Replication Protein A (RPA) is a heterotrimeric single stranded DNA-binding protein with essential roles in DNA replication, recombination and repair. In Archaea, the same function is also fulfilled by a heterotrimeric RPA. We report three crystal structures and five cryo-EM structures of Pyrococcus abyssi RPA (hereafter referred to PabRPA), in its apo form as well as bound to ssDNA. We find that archaeal and eukaryotic RPAs share a conserved heterotrimerization core, which is composed of three OB domains connected through a three-helix bundle formed by a C-terminal α-helix from each subunit.

We also collected two independent cryo-EM SPA (single-particle analysis) datasets showing multiple PabRPAs coating the ssDNA by using a poly-dT100 oligonucleotide. Interestingly, 2D class averages reveal that PabRPA dimers adopt two different conformations in the two datasets. In the second dataset, PabRPA-ssDNA complexes are more condensed, adopting a pseudo-helicoidal configuration. 2D class averages show additional density for OB-1 that connects two Tri-Cs from adjacent RPAs. Both 3D reconstructions show that two PabRPA molecules interact with each other on ssDNA through the OB-1 domain of one PabRPA that packs against the Tri-C of an adjacent PabRPA protomer particularly with its OB-4 domain. While their OB-1 domains are similarly oriented in both types of oligomeric forms, the OB-1 domain is more loosely packed to the adjacent Tri-C in the relaxed form than in the condensed one. Differences between the two DNA-bound PabRPA oligomeric forms are due to a rotation around the OB-1/OB-2 domains of the Rpa1 subunit. In the condensed PabRPA filament, this rotation brings RPA protomers closer together, compared to their position in the relaxed linear filaments observed in PabRPA and SceRPA17. Importantly, in both types of filaments, the DNA-binding groove of OB-1 is ideally located to route the ssDNA from an RPA to the other, and protect the DNA from nucleases. In P. abyssi, we observed two forms of ssDNA-RPA assemblies: a relaxed mode with PabRPA molecules arranged in tandem, and a condensed mode with RPA molecules forming a helical-like structure.

>[2x]MSVLTKDRIIEIIERKTGMSREEIEEEIRKIMEEDPYLSEQGAAALLAERLGIDLIEKEEVSLMRISELYPGMDPREVNVVGRVLKKYPPREYTRKDGSVGRVASLIIYDDSGRARVVLWDAKVSEYYNKIEVGDVIKVLDAQVKESLSGLPELHINFRARIILNPDDPRVEMIPPLEEVRVATYTRKKIKDIEAGDRFVEVRGTIAKVYRVLTYDACPECKKKVDYDEGLGVWICPEHGEVQPIKMTILDFGLDDGTGYIRVTLFGDDAEELLGVSPEEIAEKIKELEESGLTTKEAARKLAEDEFYNIIGREIVVRGNVIEDRFLGLILRASSWEDVDYRREIERIKEELEKLGVM;>[2x]MSKKRMPATRLYIKDILEGYFVKSEGDFEPNYLITKYARKVYRAKIVGTVVREPLIAEDETYGKFQVDDGTGVIWVLGFRDDTKFAKLVRKGDLVQVIGKIAEWRDDKQILVEGVSKVHPNMWILHRYETLKEKIEHIKKAKIALEIYNQYGITAKSKVIAKNKGIEEELLEVIDELYGIMMEERSIEEPMEELLEEEIPEEKEENELLEKAKEDILNILRQKRTAISRKYILKKLGDKYDEETIDDAITELLAQGEIYEPETGYYKLL;>GTGDGSEVQVRRRKPAVERKISEIREEDTRVSLIGRVIKVDKMDYMFWLDDGTGVAIIESESDLPKVGQVVRVIGRIIRNEEGIHIYAEVIQDFSDADLEALEEIRELERKLLPRLEGEIVW[2x]>MATTLPRITARVDVDTQDLLAKAAALAGMSSINSFVLNAAIEKAKQVIEREQALKLSQADAVLLMEALD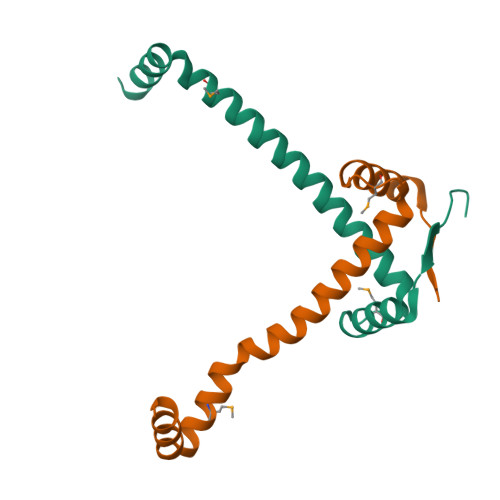NPAVVNAKLKLASERYESKTQ[2x]> GPGTRTGRLKKPFVKVEDMSQLYRPFYLQLTNMPFINYSIQKPCSPFDVDKPSSMQKQTQVKLRIQTDGDKYGGTSIQLQLKEKKKKGYCECCLQKYEDLETHLLSEQHRNFAQSNQYQVVDDIVSKLVFDFVEY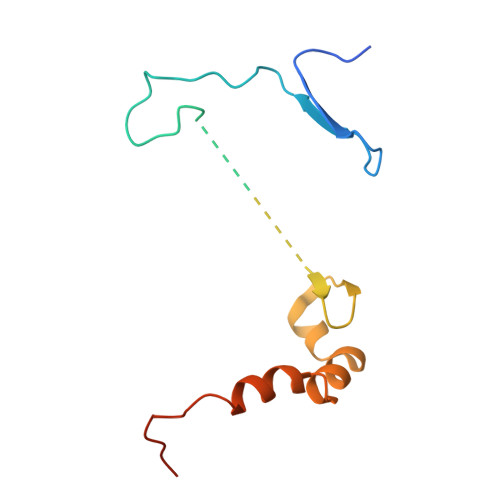EKDTPKKKR> MSSHHHHHHSSGLVPRGSHMTDQGLEGSNPVDLSKHPSGI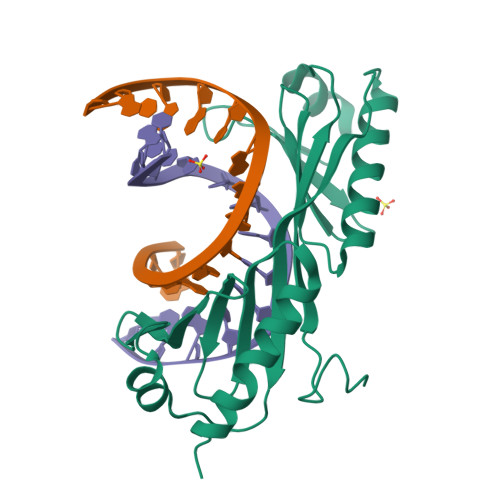VPTLQNIVSTVNLDCKLDLKAIALQARNAEYNPKRFAAVIMRIREPKTTALIFASGKMVCTGAKSEDFSKMAARKYARIVQKLGFPAKFKDFKIQNIVGSCDVKFPIRLEGLAYSHAAFSSYEPELFPGLIYRMKVPKIVLLIFVSGKIVITGAKMRDETYKAFENIYPVLSEFRKIQQ>[2x]EAEFPTDGVDIYFGMPGEISEHEGFLRAKMDLEERRMR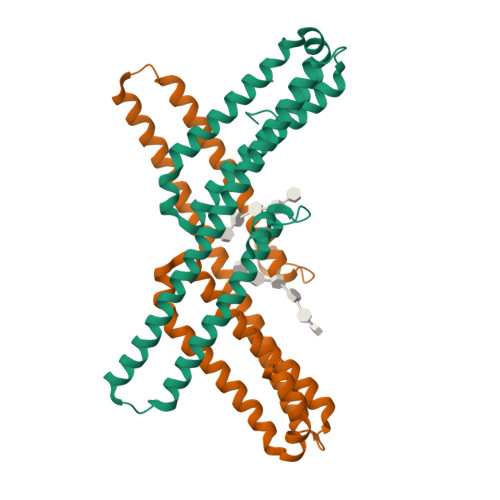QINEVMREWAMADNQSKNLPKADRQALNEHFQSILQTLEEQVSGERQRLVETHATRVIALINDQRRAALEGFLAALQADPPQAERVLLALRRYLRAEQKEQRHTLRHYQHVAAVDPEKAQQMRFQVHTHLQVIEERVNQSLGLLDQNPHLAQELRPQIQELLHSEHLGPSEL>AAVLQQVLERTELNKLPK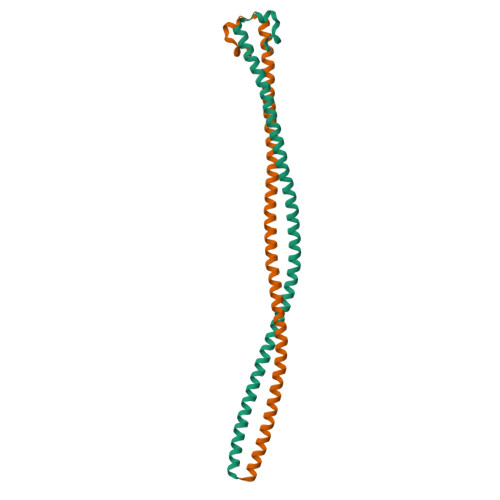SVQNKLEKFLADQQSEIDGLKGRHEKFKVESEQQYMEIEKRLSHSQERLVNETRECQSLRLELEKLNNQLKALTEKNKELEIAQDRNIAIQSQMTRTKEELEAEKRDLIRTNERLSQELEYLT[2x]> GAPATVTEQGEDITSKKDRGVLKIVKRVGNGEETPLIG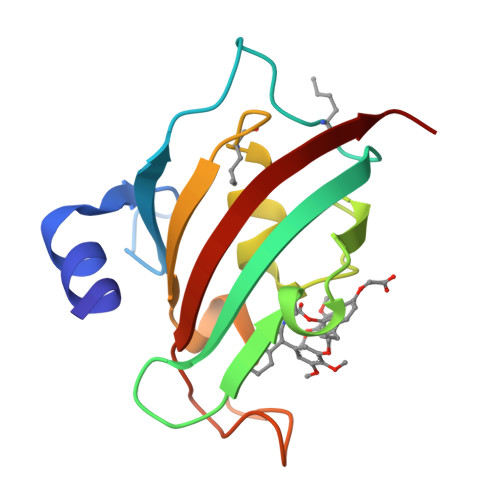DKVYVHYKGKLSNGKKEDSSHDRNEPFVFSLGKGQVIKAWDIGVATLKKGEIAHLLIKPEYAYGSAGSLPKIPSNATLFFEIELLDFKGE>HHHHHHDSGLVPRGSHMHGNHTHWGYTGHDSPESWGNLSEEFRLCSTGKNQSPVNITETVSGKLPAIKVNYKPSMVDVENNGHTIQVNYPEGGNTLTVNGRTYTLKQFHFHVPSENQIKGRTFPMEAHFVHLDENKQPLVLA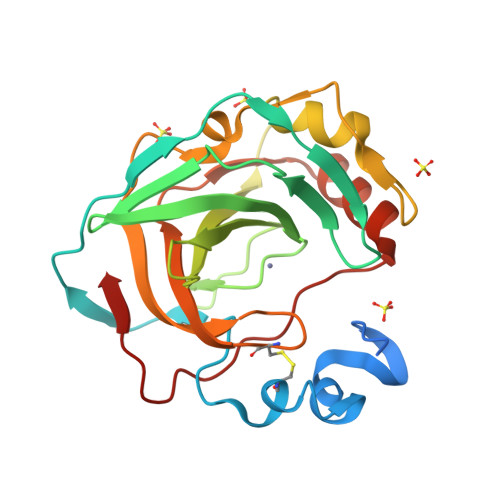VLYEAGKTNGRLSSIWNVMPMTAGKVKLNQPFDASTLLPKRLKYYRFAGSLTTPPCTEGVSWLVLKTYDHIDQAQAEKFTRAVGSENNRPVQPLNARVVIE[4x]>MFNQFNPLVYTHGGKLERKSKKDKTASKVFEEFGVMEAYNCWKEASLCIQQRDKDSVLKLVAALNTYKDAVEPIFDSRLNSAQEVLQPSILEEFFEYLFSRIDSIVGVNIPIRHPAKGYLSLSFNPHNIETLIQSPEYTVRAKDHDFIIGGSAKLTIQGHGGEGETTNIVVPAVAIECKRYLERNMLDECAGTAERLKRATPYCLYFVVAEYLKLDDGAPELTEIDEIYILRHQRNSERNKPGFKPNPIDGELIWDLYQEVMNHLGKIWWDPNSALQRGKV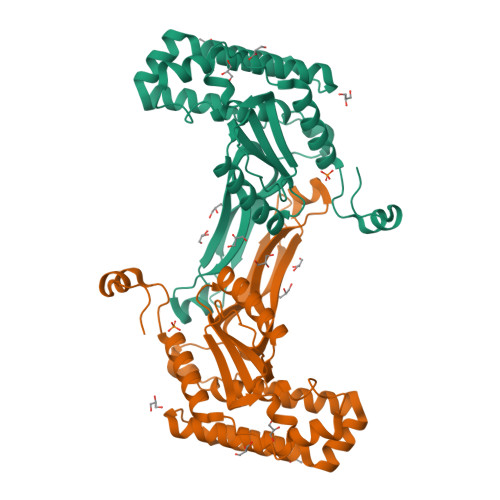FNRP[3x]Glutamine synthetases (GS) are central enzymes essential for the nitrogen metabolism across all domains of life. Accordingly, GS present across all domains of life plays a central role in cellular N assimilation under low N availability. GlnA1 is not covalently modified in response to N availability and thus represents an Iα-type-GS. It has been proposed, that GlnA1 is directly activated under N starvation by the high intracellular concentrations of the metabolite 2-OG.

The 2.39 Å cryo-EM structure of the dodecameric complex in the presence of 12.5 mM 2-OG demonstrated that 2-OG is binding between two monomers. The detailed structural analysis uncovered that GlnA1 assembles into a dodecamer characterized by stacked hexamer rings. The dodecameric arrangement is achieved through two distinct interfaces, the hexamer interfaces and inter-hexamer interfaces. A closer inspection of the density reveals the density for the bound 2-OG at an allosteric site localized at the interface between two GlnA1 protomers in vicinity of the GlnA1 catalytic site. R172’ and S189’ coordinate the γ-Carboxy-group. Notably, F24 stabilizes the 2-OG via stacking with its phenyl ring. R87' and its loop undergo a dramatic flip to coordinate 2-OG and D170 of helix α3 (residues 167–181). Notably, helix α3 shifts forward, causing F184 to flip over and facilitate a T-shaped aromatic interaction with F202. The resulting pull on F202 causes F204 to flip, allowing π-stacking with the purine moiety of ATP. The conformation of our 2-OG-bound dodecamer resembled the transition state conformation (ADP-Met-Sox-bound complex) reported by Schumacher et al., even though in our case no ATP was added.

>[12x]VQMKKCTTKEDVLEAVKERDVKFIRTQFTDTLGIIKSWAIPAEQLEEAFENGVMFDGSSIQGFTRIEESDMKLALDPSTFRILPWRPATGAVARILGDVYLPDGNPFKGDPRYVLKTAIKEAEKMGFSMNVGPELEFFLFKLDANGNPTTELTDQGGYFDFAPLDRAQDVRRDIDYALEHMGFQIEASHHEVAPSQHEIDFRFGDVLCTADNVVTFKYVVKSIAYHKGYYASFMPKPLFGVNGSGMHSNQSLFKDGKNVFYDPDTPTKLSQDAMYYIGGLLKHIREFTAVTNPVVNSYKRLVPGYEAPVYISWSAQNRSSLIRIPATRGNGTRIELRCPDPACNPYLAFALMLRAGLEGIKNKIDPGEPTNVNIFHLSDKEREERGIRSLPADLKEAIDEMKGSKFVKEALGEHVFSHYLCAKEMEWDEYKAVVHPWELSRYLSML>[2x]MLRFVTKNSQDKSSDLFSICSDRGTFVAHNRVRTDFKFDNLVFNRVYGVSQKFTLVGNPTVCFNEGSSYLEGIAKKYLTLDGGLAIDNVLNELRSTCGIPGNAVASHAYNITSWRWYDNHVALLMNMLRAYHLQVLTEQGQYSAGDIPMYHDGHVKIKLPVTIDDTAGPTQFAWPSDRSTDSYPDWAQFSESFPSIDVPYLDVRPLTVTEVNFVLMMMSKWHRRTNLAIDYEAPQLADKFAYRHALTVQDADEWIEGDRTDDQFRPPSSKVMLSALRKYVNHNRLYNQFYTAAQLLAQIMMKPVPNCAEGYAWLMHDALVNIPKFGSIRGRYPFLLSGDAALIQATALEDWSAIMAKPELVFTYAMQVSVALNTGLYLRRVKKTGFGTTIDDSYEDGAFLQPETFVQAALACCTGQDAPLNGMSDVYVTYPDLLEFDAVTQVPITVIEPAGYNIVDDHLVVVGVPVACSPYMIFPVAAFDTANPYCGNFVIKAANKYLRKGAVYDKLEAWKLAWALRVAGYDTHFKVYGDTHGLTKFYADNGDTWTHIPEFVTDGDVMEVFVTAIERRARHFVELPRLNSPAFFRSVEVSTTIYDTHVQAGAHAVYHASRINLDYVKPVSTGIQVINAGELKNYWGSVRRTQQGLGVVGLTMPAVMPTGEPTAGAAHEELIEQADNVLVE

S. cerevisiae, a genetically well-described system, harbors in its genome an endogenous virus known as L-A virus, a member of the Totivirus family, and its discovery was the main starting point of research on yeast virology. The L-A virus contains a single 4.6 kb double-stranded RNA (dsRNA), encoding for a capsid protein (Gag), and the viral RNA-dependent RNA polymerase fusion protein (Gag/Pol).

To isolate complexes of similar molecular weight within the native cell extract, we performed size exclusion chromatography (SEC) and reproducibly collected the resulting fractions in less than 8 h from harvesting yeast cells (“Methods”). After SEC, we vitrified fractions 5 and 6 that include megadalton (MDa) assemblies (orange dotted line). In the acquired cryo-EM micrographs, large unperturbed complexes are visible, including fatty acid synthase (FAS)44 and polysomes as well as prominent circular signatures. To first explore this signature, we collected 7011 movies at a pixel size of 1.57 Å and performed image analysis of the derived spherical signatures, resulting in an icosahedrally averaged cryo-EM map at 3.77 Å resolution (FSC = 0.143) in which an initial backbone trace could be built. Simultaneously, we used ModelAngelo47, an automatic model-building tool, in its de novo mode, enabling us to construct an atomic model within the EM density. The patches generated in this process were then compared against the “non-redundant protein sequence (nr)” database, a task executed using the blastp suite. Mass spectrometry (MS)-based protein identification of the fractionated cell extract verified the abundance of the L-A helper virus (Gag, Gag/Pol), and also the presence of the L-BC virus, albeit with lower abundance, after adding these endogenous protein sequences to the available yeast proteome (UP000002311)22. Compared to other studies, we succeeded in (a) mildly reducing sample complexity and rapidly retrieving L-A virus in yeast cell extracts directly amenable for cryo-EM; (b) identifying unambiguously the L-A virus using the high-resolution features of the calculated cryo-EM map by Cα-trace model building in a supervised and unsupervised manner; and (c) probing the environment and components of the L-A virus by quantitative mass spectrometry.>GGPIPYPVGNLLHTAPCGFIVTDAVEPDQPIIYVNTVFEMVTGYRAEEVLGRNCRFLQCRGPFAKRRHPLVDSMVVSEIRKCIDEGIEFQGELLNFRKDG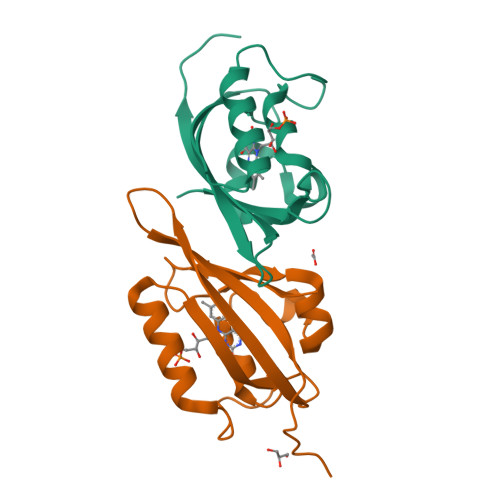SPLMNRLRLTPIYGDDDTITHIIGIQFFIETDIDLGP[4x]> MAAPAAEAPLSHVQQALAELAKPKDDPTRKHVCVQVAPAVRVAIAETLGLAPGATTPKQLAEGLRRLGFDEVFDTLFGADLTIMEAGSELLHRLTEHLEAHPHSDEPLPMFTSCCPGWIAMLEKSYPDLIPYVSSCKSPQMMLAAMVKSYLAEKKGIAPKDMVMVSIMPCTRKQSEADRDWFCVDADPTLRQLDHVITTVELGNIFKERGINLAELPEGEWDNPMGVGSGAGVLFGTTGGVMEAALRTAYELFTGTPLPRLSLSEVRGMDGIKETNITMVPAPGSKFEELLKHRAAARAEAAAHGTPGPLAWDGGAGFTSEDGRGGITLRVAVANGLGNAKKLITKMQAGEAKYDFVEIMACPAGCVGGGGQPRSTDKAITQKRQAALYNLDEKSTLRRSHENPSI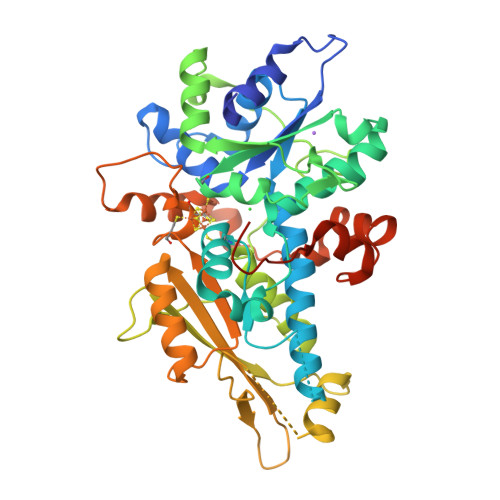RELYDTYLGEPLGHKAHELLHTHYVAGGVEEKDEKKSAWSHPQFEK O-glycosylation of the protein CST1 by the mucin-type O-glycosyltransferase T. gondii (Txg) GalNAc-T3 influences cyst wall rigidity and stability. The strict glycopeptide-preferring enzyme TxgGalNAc-T3 then adds GalNAc to acceptor Thr one position N-terminal to existing Thr-O-GalNAcs and is predicted to sequentially O-glycosylate Thr rich repeats within the mucin domain of CST1. The structures reveal a unique GalNAc binding pocket that dictates the substrate preference of TxgGalNAc-T3, which is coupled to a 2nd metal binding site that is strictly conserved among apicomplexan homologs.

We then verified the substrate preference of TxgGalNAc-T3 for endogenous T. gondii cyst wall proteins using peptides and glycopeptides from CST1 and SRS13. TxgGalNAc-T3 does not readily modify the unglycosylated SRS13.1 peptide, as predicted. Surprisingly, there is diminished activity for the C-terminal mono-glycopeptide SRS13.3, while activity for the SRS13.4 di-glycopeptide is ~1.5-fold lower than the SRS13.2 mono-glycopeptide despite the availability of two potential acceptor sites, suggesting that either the C-terminal acceptor site or proximal amino acids are inhibiting enzymatic activity. We observe similar sequential and gradually decreasing glycosylation efficiency for the Muc5AC glycopeptides and SRS13.2 after 90 mins. To investigate the basis of the substrate specificity and function of TxgGalNAc-T3, we solved the x-ray co-crystal structures of TxgGalNAc-T3 in complex with Mn2+, a non-hydrolysable form of UDP-GalNAc (UDP-2-(acetylamino)−4-F-D-galactosamine disodium salt, UDP-GalNAc-F) and each of the following glycopeptides: CST1.4, Muc5AC-3,13, Muc5AC-3, Muc5AC-13, and SRS13.2 from 2.2-2.9 Å resolution. We could not model the peptide substrate in the structure containing Muc5AC-13 due to unresolvable electron density, and we only observe weak density for Thr-O-GalNAc in the SRS13.2 structure. Overall, the lack of density for the peptide backbone or Thr-O-GalNAc at the C-terminal ends of the glycopeptides suggests a lack of strong interactions with the catalytic or lectin domain of TxgGalNAc-T3.

>[2x]GARDVQEGVSSFEESGGAQLPPRVHALEVLEGAGPGRLHGRLGIKPDGQPGYTRAPSPPTDLSMPQALARGGGFNLYLSDHLELDRTAPDARHASCRQLHYDLSTLPKASVIIVFYNEPFSTLMRSVHSVLNGTPPQILEELILVDDGSTLPYIREDGNQQLVEYLKLLPAKVRLIRNEVRKGIVGARMKGIRASRAPIFAILDSHIEVSPQWLEPLLLRIKEDSRRVVMPQIDGIDAETFKHIAGGIGCKLGFLWKLMEHSYEGHQTARLPPEERQPSPTDFQTSPAMAGGLFAANKAFFFDVGAYDEDFQFWGTENLELSFRLWQCGGVLECAPCSRVYHIFRKGGSGYSSPGDSITINKMRTMLWMDEYADLAWRVIGKPRVNYRPESLEKRREWRKRKGCKSFRWFMENVFPEGDVVTLDDVPYLGPLRNDKIGMCLDNMGWASPGHAVGLEYCHGGDTQTFMFFRKVGHVMPVNDDEACLQPSGRLDWCRGTAQFWWDFTSSGQLMFRETKQCLSAFGRKLRMVECDDTDPYQIWSWTAYNPPDTFTFPSVSRSIRSG;> PETTTVAPPAKTQPETTTV Hearing sensitivity in mammals is sharply tuned by a cochlear amplifier associated with electromotile length changes in outer hair cells. These changes are driven by prestin (SLC26A5), a member of the SLC26 anion transporter family, which converts voltage-dependent conformational transitions into cross-sectional area changes, affecting its footprint in the lipid bilayer. Prestin belongs to the SLC26 family of anion transporters yet is the only member capable of displaying electromotility. Prestin’s voltage-dependent conformational changes are driven by the putative displacement of residue R399 and a set of sparse charged residues within the transmembrane domain, following the binding of a Cl− anion at a conserved binding site formed by the amino termini of the TM3 and TM10 helices. Recent structures determined by cryo-electron microscopy (cryo-EM) have sampled prestin’s conformational space under various anionic environments and located the anion-binding site at the electrostatic gap between the amino termini of TM3 and TM10 helices.

In a HEPES-based buffer, prestin’s NLC shifts to depolarized potentials, associated to a more expanded state at 0 mV that is coupled to low anion affinity. Based on the above studies and the large size of HEPES anions, we assumed minimal binding of HEPES anions to prestin and hence associated HEPES condition to a putative apo state in this study. We associate the HEPES solvent condition to an apo state as the HEPES anion is too big to fit into the chloride site and prestin has a right-shifted NLC, To investigate further whether HEPES anion binds, we determined the structure of prestin in the HEPES-based buffer using cryo-EM. Our initial attempt to solve the structure in the complete absence of Cl− was unsuccessful due to sample aggregation under cryogenic conditions. Aggregated particles were greatly reduced in the presence of 1 mM Cl−, and we were able to solve the structure of GDN-solubilized prestin in 1 mM Cl−, containing 190 mM HEPES, at a nominal resolution of 3.4 Å. Surprisingly, under these conditions prestin adopted a ‘compact’ conformation, virtually identical to the previously reported Cl−-bound ‘Up’ state, displaying a clear density at the anion-binding site. This density is incompatible with the placing of a HEPES molecule, and we reason it to be a small population of Cl−-bound prestin resulting from a weak Cl− affinity (e.g., EC50 = 6 mM11 implies 17% bound). At physiologically relevant low Cl− concentration (1.5–4 mM), prestin’s binding site is likely to be only partially folded.

>[2x]MDHVEETEILAATQRYYVERPIFSHPVLQERLHKKDKISESIGDKLKQAFTCTPKKIRNIIYMFLPITKWLPAYRFKEYVLGDIVSGISTGVLQLPQGLAFAMLAAVPPVFGLYSSFYPVIMYCFFGTSRHISIGPFAVISLMIGGVAVRLVPDDIVIPGGVNATNSTEARDALRVKVAMSVTLLTGIIQFCLGVCRFGFVAIYLTEPLVRGFTTAAAVHVFTSMLKYLFGVKTKRYSGIFSVVYSTVAVLQNVKNLNVCSLGVGLMVFGLLLGGKEFNERFKEKLPAPIPLEFFAVVMGTGISAGFSLHESYNVDVVGTLPLGLLPPANPDTSLFHLVYVDAIAIAIVGFSVTISMAKTLANKHGYQVDGNQELIALGLCNSTGSLFQTFAISCSLSRSLVQEGTGGKTQLAGCLASLMILLVILATGFLFESLPQAVLSAIVIVNLKGMFMQFSDLPFFWRTSKIELTIWLTTFVSSLFLGLDYGLITAVIIALMTVIYRTQSPSYIVLGQLPDTDVYIDIDAYEEVKEVPGIKIFQINAPIYYANSDLYSSALKRKTGVNPAFILGARRKAMKKYAKEVGNANMANATVVKVDAEVDAEDGTKPEEEEDEIKYPPIVTKSTLPEELQRFMPPGDNVHTIILDFTQVNFMDSVGVKTLAGIVKEYGDVGIYVYLAGCSAQVVSDLTQNQFFENPALLDLLFHSIHDAVLGSQVREALAEQEATAAPPQEDSEPNATPEA> MEKPAEQVHLSGPTMGTTYNIKYIQQPGIADSKTLQTEIDRLLEEVNDQMSTYRKDSELSRFNQHTSSEP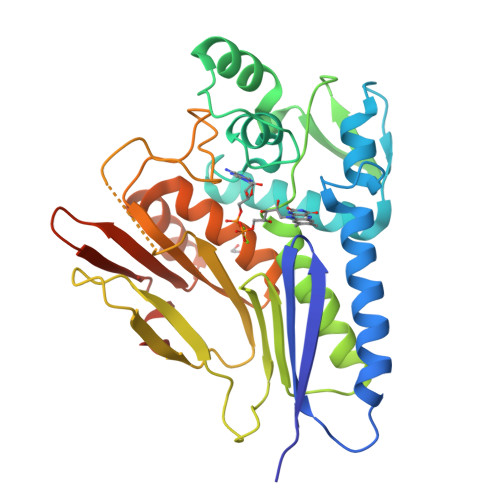FAVSTQTLTVVKEAIRLNGLTEGALDVTVGPLVNLWGFGPEARPDVVPTDEELNARRAITGIEHLTIEGNTLSKDIPELYVDLSTIAKGWGVDVVADYLQSQGIENYMVEIGGEIRLKGLNRDGVPWRIAIEKPSVDQRSVQEIIEPGDYAIATSGDYRNYFEQDGVRYSHIIDPTTGRPINNRVVSVTVLDKSCMTADGLATGLMVMGEERGMAVAEANQIPVLMIVKTDDGFKEYASSSFKPFLSKGGGGHHHHHH>[2x]ALYEDPPDQKTSPSGKPATLKICSWNVDGLRAWIKKKGLDWVKEEAPDILCLQETKCSENKLPAELQELPGLSHQYWSAPSDKEGYSGVGLLSR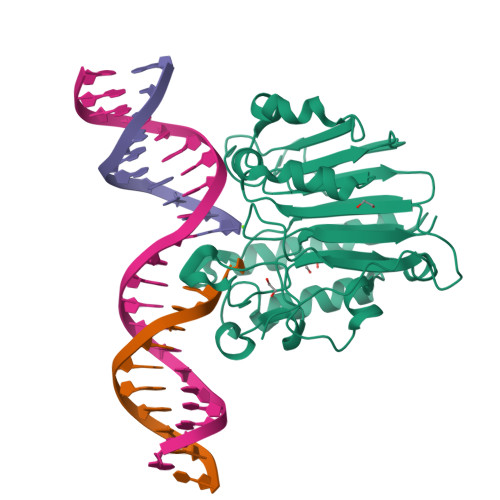QCPLKVSYGIGEEEHDQEGRVIVAEFDSFVLVTAYVPNAGRGLVRLEYRQRWDEAFRKFLKGLASRKPLVLCGDLNVAHEEIDLRNPKGNKKNAGFTPQERQGFGELLQAVPLADSFRHLYPNTPYAYTFWTYMMNARSKNVGWRLDYFLLSHSLLPALCDSKIRSKALGSDHCPITLYLAL>EVSQDLFNQFNLFAQYSAAAYCGKNNDAPAGTNITCTGNACPEVEKADATFLYSFEDSGVGDVTGFLALDNTNKLIVLSFRGSRSIENWIGNLNFDLKEINDICSGCRGHDGFTSSWRSVADTLRQKVEDAVREHPDYRVVFTGHSLGGALATVAGADLRGNGYDIDVFSYGAPRVGNRAFAEFLTVQTGGTLYRITHTNDIVPRLPPREFGYSHSSPEYWIKSGTLVPVTRNDIVKIEGIDATGG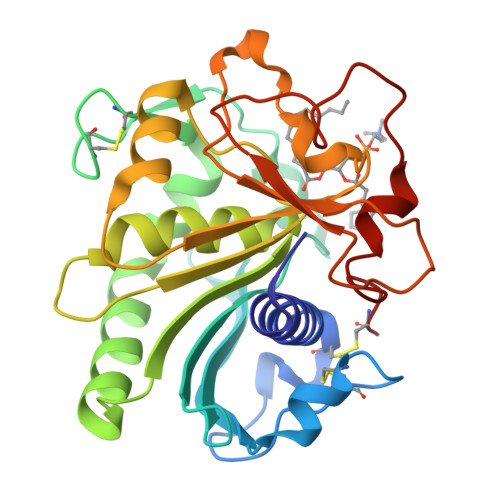NNQPNIPDIPAHLWYFGLIGTCL[3x]> MGSSHHHHHHSSGLVPRGSHISFDTSSNGITDAELAPINNAINDAIVSNRDNKLKPSEEKIIKETEKKIEEKIIIPPAKKEEKIEAAKPIPKPVVRKPETKITSPKITRRKQTITIAGIEVEAEIEGPPGFVTHQRDKDRKISNPTKPYQNHTVNKILSVKVTDKLKEQVAKDALSGGNGYDEGVGLFNNSIFNVFKEEFNSGKELNDILSSLESVARQNSGAFQNTL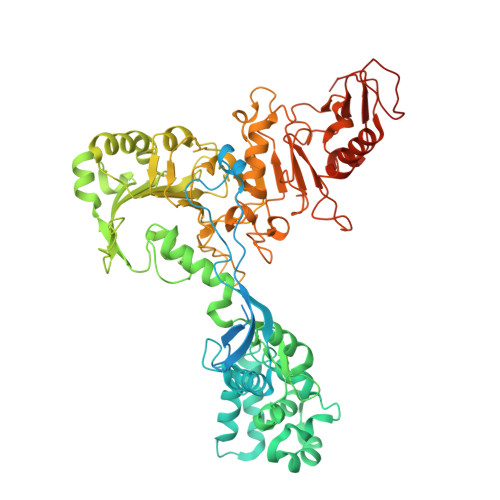ERYKKMLDSNNVINFLKSEAQKEYPKLKSKFQTKNQEYIWLIANLDQSKFTKIASTSEKYLEKGLTISPRSAFINEAGEIDSNGWGPPDEYNTVTSRLRRDNSEYRVFDYDEYYSRSSDRIANGTYPGWVKEDVSEPYSKKYNFKASDGIRFSKLERINPNPAKGKLNSGLVLDLDVSNDEAYRRSKELIEKLQKDGEQITSYRIKNMGEKNSDQAFKDILGALPKDIQQLELFFSDKATNTASLIALENKNIKELSLYTSGNSLKKAWSYNPLALRNTTWINTIDYNVSAEYSSHDKITTRITFNTLAFDQEDFSNGSYERINDGLRMVYYARNNEPFFQGGHGPGLEPDKKLGQNSYPTGLDFSRVTGIKSLKGLRFDDDLDTSNEPRKITELTLYNNESYFEISSDELNEANLQHLSTGEGNPEKPKIHFSNGNNTTSIRISGKTLLSDEGRRNLDKYFEYNESLRNSGKQIQIPNGSDELKKQLEGWGYKVSTASDRSFT>GSKVYDPEQRKRMITGPQWWARCKQMNVLDSFINYYDSEKHAENAVIFLHGNATSSYLWRHVVPHIEPVARCIIPDLIGMGKSGKSGNGSY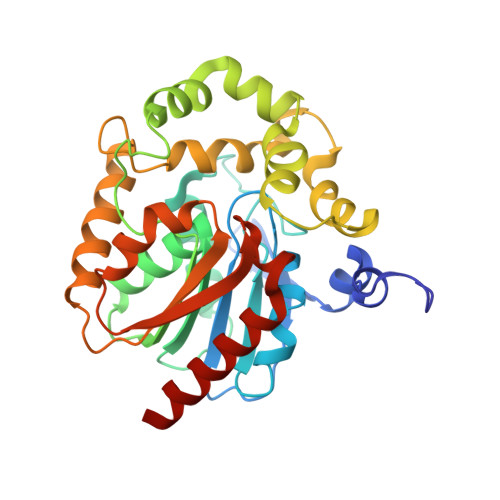RLLDHYKYLTAWFELLNLPKKIIFVGHDWGAALAFHYAYEHQDRIKAIVHMESVVDVIESWDEWPDIEEDIALIKSEEGEKMVLENNFFVETVLPSKIMRKLEPEEFAAYLEPFKEKGEVRRPTLSWPREIPLVKGGKPDVVQIVRNYNAYLRASDDLPKLFIESDPGFFSNAIVEGAKKFPNTEFVKVKGLHFLQEDAPDEMGKYIKSFVERVLKNEQ[2x]>[4x]RMVDLPVLQPRLCTHARWPAPIYGLLVDPSLPSNPQWQNGRVHVDGTLLGTTPVSGSWVSCFAAEAAYEFQSGTGEVATFTLIEQDGSAYVPGDRAAPLGYPDFS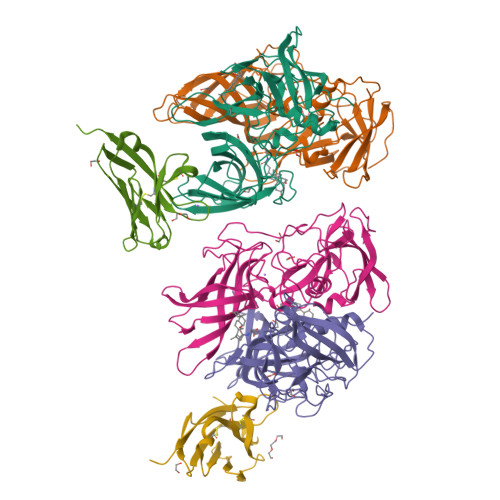GQLEIEVQTETTKTGDKLKVTTFEMILGPTTNVDQAPYQGRVYASLTAVASLDLVDGRVRAVPRSIYGFQDVIPEYNDGLLVPLAPPIGPFLPGEVLLRFRTYMRQLDTADAAAEAIDCALPQEFISWFASNAFTVQSDALLLRYRNTLTGQLLFECKLYSEGYIALSYSGSGPLTFPTDGFFEVVSWVPRLFQLASV;>[2x]EDPVTGPEEVSGQEQGSLTVQCRYTSGWKDYKKYWCQGVPQRSCKTLVETDASEQLVKKNRVSIRDNQRDFIFTVTMEDLRMSDAGIYWCGITKGGLDPMFKVTVNIGPVP>[2x]MKKLFLVFWWHMHQPLYREPYTGEYLLPWTFFHAVKDYYDMPAYLKDFEIKLNFNLTPVLIDQIQEYAQGKAKDVFLEAIR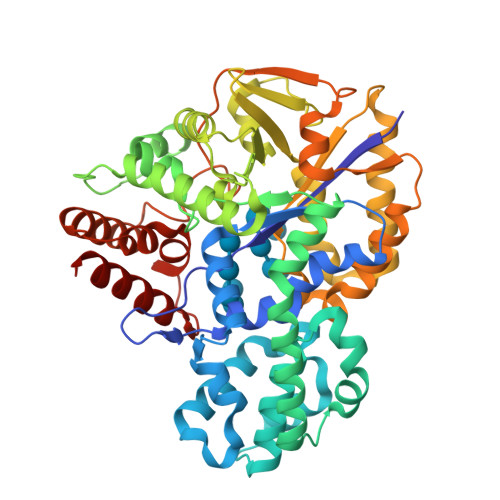KDPDDLEKEEVEKLIEFTKLNYEKPIYRFERIRELMNKEKLNREELLDLQTLNLLAWCGRTLRKDLKDLLNKGRNYTQEEKEYVLNKYFEIIKKTLSIYREIKEEGKGSVSTSPYYHPLIPILLNPNCVYETTPNVKIPDFAVSFREDASKHVELAKEKYFEIFGEHPVYMWPPQASVSNEALELYYEKGINMLATDEVILKNSVERASPYLRYYFRELISVFFRDKTLSDLIGFSYHAWNAEDAVRDFIGRLKKIHESVDFQPVVFVVLDGENCWEYYEENGIPFLEKLYSTLEKEEWIETLTLEEAMRKEDVKTEVIESVKAGTWFDGNFLKWIGNKEKNEYWKILIEAKKKAKNDYILVAEGSDWFWWQGEEKAPFVEVFDKLFRSFVRRAQE> MSSTTSTAAGAAAEVESVVDLRGMWIGLAVLNVFYLIVRIYEQVFGWRAGLDSFAPEFQTYWMSILWTEIPLELVSGLGLAGYLWKTRDRNVDAVAPREEMRRLVVLVQWLVVYGIAIYWGASFFTEQDGAWHMTVIRDTDFTPSHIIEFYMSYPIYSVIAVGAFFYAKTRIPYFAHGYSLAFLIV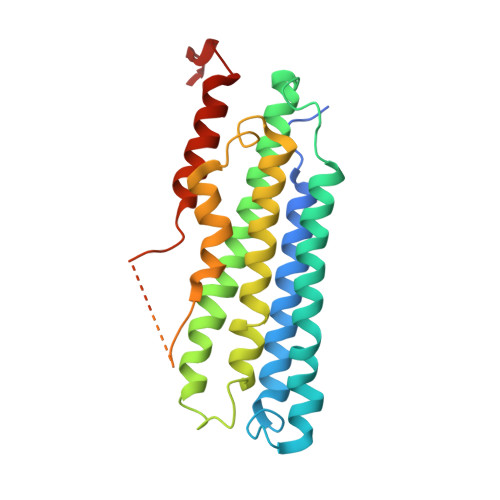AIGPFMIIPNVGLNEWGHTFWFMEELFVAPLHWGFVFFGWMALGVFGVVLQILGRIHALIGKEGVALLTE[(3~{R})-3-phenyl-1-(phenylmethyl)pyrrolidin-3-yl]methanol 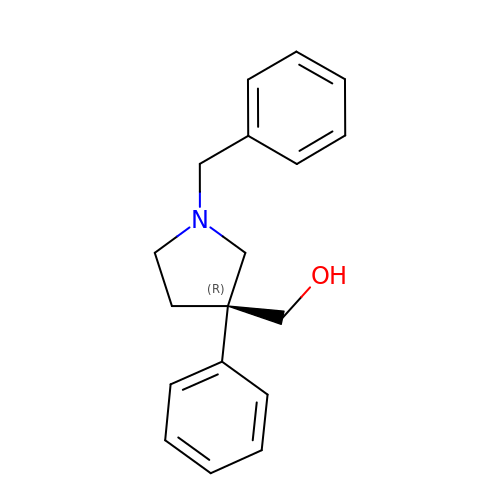| C18 H21 N O | SEKWWCPJXPJZKJ-GOSISDBHSA-N> GAMGSTSLEPTSTLVRVRKSAATLGIAIEGGANTRQPLPRIVTIQRGGSAHNCGQLKVGHVILEV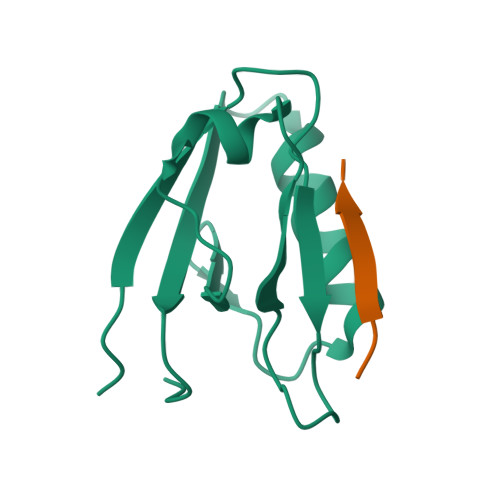NGQTLRGKEHKEAARIIAEAFKTKERDYIDFLVTEFNVML;> TAPQWVPVSWVY>[2x]MSGRRELCTPLRTIMTPGPVEVDPRVLRVMSTPVVGQFDPAFTGIMNETMEMLRELFQTKNRWAYPIDGTSRAGIEAVLASVIEPEDDVLIPIYGRFGYLLTEIAERYGANVHMLECEWGTVFDPEDIIREIKKVKPKIVAMVHGETSTGRIHPLKAIGEACRTEDALFIVDAVATIGGCEVKVDEWKIDAAIGGTQKCLSVPSGMAPITYNERVADVIAARKKVERGIATQADRAAL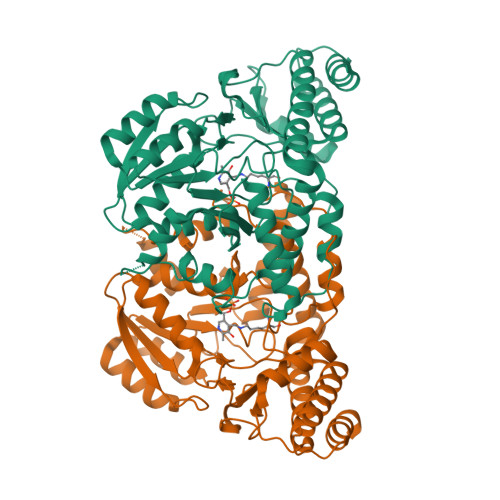SGNRPITSNYFDLSQLEDYWSERRLNHHTEATTMLYALREGVRLVLEEGLETRFERHRHHEAALAAGIKAMGLRLFGDDSCKMPVVTCVEIPGGIDGESVRDMLLAQFGIEIASSFGPLAGKIWRIGTMGYSCRKENVLFVLAGLEAVLLRHNAGIEAGKALQAALDVYENAGRQAAV> RKKQDPPVTHDLRVSLEEIYSGCTKKMKISHKRLNPDGKSIRNEDKILTIEVKKGWKEGTKITFPKEGDQTSNNIPADIVFVLKDKPHNIFKRDGSDVIYPARISLREALCGCTVNVPTLDGRTIPVVFK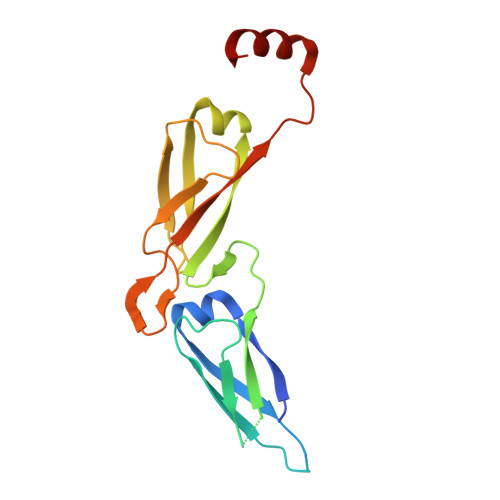DVIRPGMRRKVPGEGLPLPKTPEKRGDLIIEFEVIFPERIPQTSRTVLEQVLPI(2S)-N-[4-[1-METHYL-3-(1-METHYLPYRAZOL-4-YL)INDOL-5-YL]OXYPHENYL]PYRROLIDINE-2-CARBOXAMIDE | C24 H25 N5 O2 | 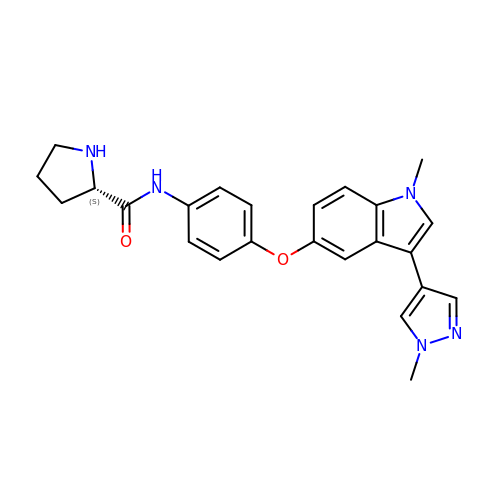JTIOFEOXCFFWJI-QFIPXVFZSA-N>MTAVQLIVGLGNPGPEYDQTRHNAGALFVERLAHAQGVSLVADRKYFGLVGKFSHQGKDVRLLIPTTYMNRSGQSVAALAGFFRIAPDAILVAHDELDMPPGVAKLKTGGGHGGHNGLRDIIAQLGNQNSFHRLRLGIGHPGHSSLVSGYVLGRAPRSEQELLDTSIDFALGVLPEMLAGDWTRAMQK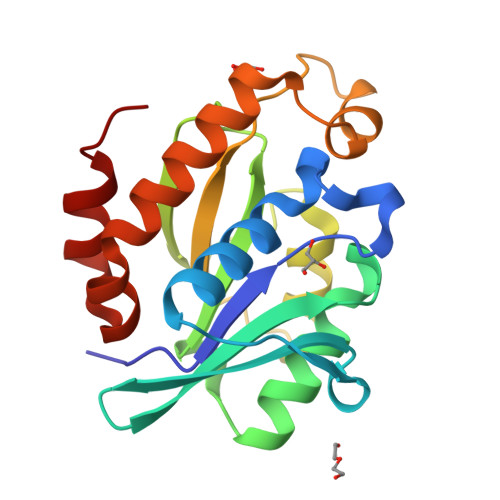LHSQKA[2x]>MIRISNKIKTLLAMLSFVQVTSGCDATVQDIIIDTDPGVEIGNNDYYTWCKETLSVIDKDLKISGTHSYYENQDRSQVSFIWGNIFLLYTYTEGISLSKSEWSDALMNCFLNFDNYWHPNYKGIAGYATLPTSAEKVPDRFYDENGWTAIGLCDAYLATQNNSYLEKAKGALAFSLSGEDNVLGGGIYFQETFVSLPVQKNTICSAVTMLSCMKLYEITQDRQYLDAAIRINDWTVENLLDKSDNLLWDAKMVADGSVNTQKWSYNAGFMIRSWLKMYQATKDEKYLSQAKA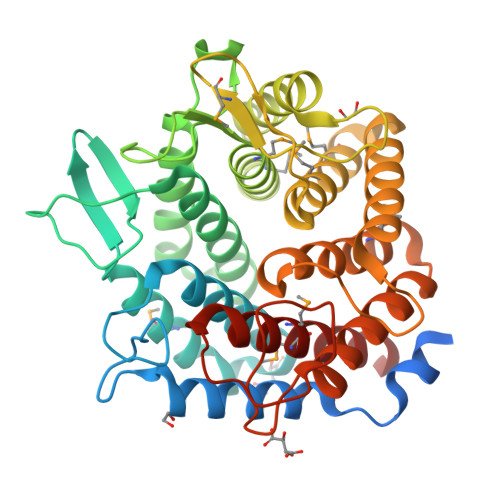TLASSEAKWYNSINGALNDPGYFAFSIIDSWFDMYDTDKNTVWLTKAFHAINFIHNKLRDGNGRYPEHWGTPTTSNLEKYDLRFSTVAAYMYMRAANYKRILND[2x]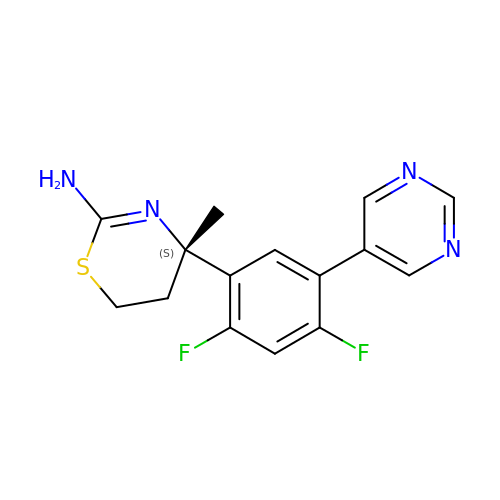(4S)-4-[2,4-difluoro-5-(pyrimidin-5-yl)phenyl]-4-methyl-5,6-dihydro-4H-1,3-thiazin-2-amine | C15 H14 F2 N4 S | MJQMRGWYPNIERM-HNNXBMFYSA-N> MLKVNEFETDTDLRGNINYLFNDEANVVYTYDGTESDLLQNVNEVSKYIEHHMDYQRPRLKVLSDYYEGKTKNLVELTRRKEEYMADNRVAHDYASYISDFINGYFLGNPIQYQDDDKDVLEAIEAFNDLNDVESHNRSLGLDLSIYGKAYELMIRNQDD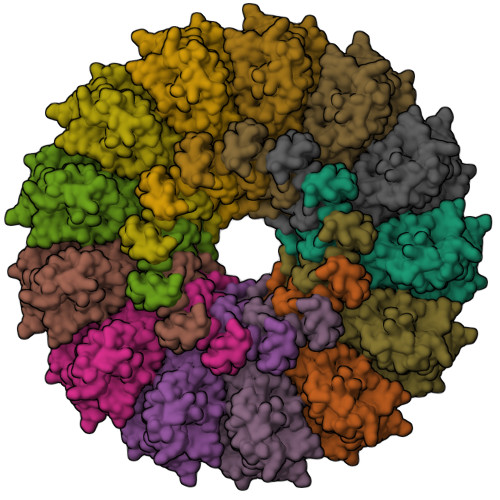ETRLYKSDAMSTFIIYDNTVERNSIAGVRYLRTKPIDKTDEDEVFTVDLFTSHGVYRYLTNRTNGLKLTPRENSFESHSFERMPITEFSNNERRKGDYEKVITLIDLYDNAESDTANYMSDLNDAMLLIKGNLNLDPVEVRKQKEANVLFLEPTVYVDAEGRETEGSVDGGYIYKQYDVQGTEAYKDRLNSDIHMFTNTPNMKDDNFSGTQSGEAMKYKLFGLEQRTKTKEGLFTKGLRRRAKLLETILKNTRSIDANKDFNTVRYVYNRNLPKSLIEELKAYIDSGGKISQTTLMSLFSFFQDPELEVKKIEEDEKESIKKAQKGIYKDPRDINDDEQDDDTKDTVDKKE> FTMEFPFDVDALFPERITVLDQHLRPPARRPG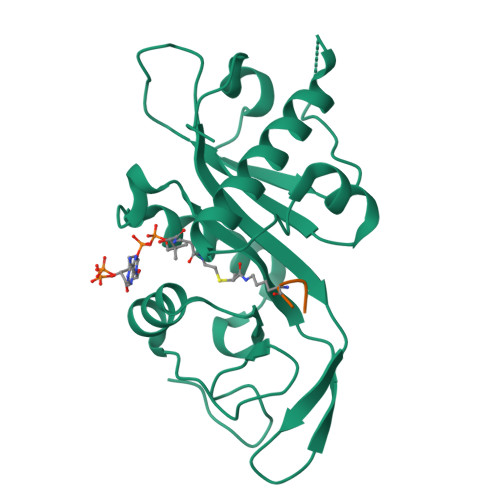TTTPARVDLQQQIMTIIDELGKASAKAQNLSAPITSASRMQSNRHVVYILKDSSARPAGKGAIIGFIKVGYKKLFVLDDREAHNEVEPLCILDFYIHESVQRHGHGRELFQYMLQKERVEPHQLAIDRPSQKLLKFLNKHYNLETTVPQVNNFVIFEGFFAHQHPP>[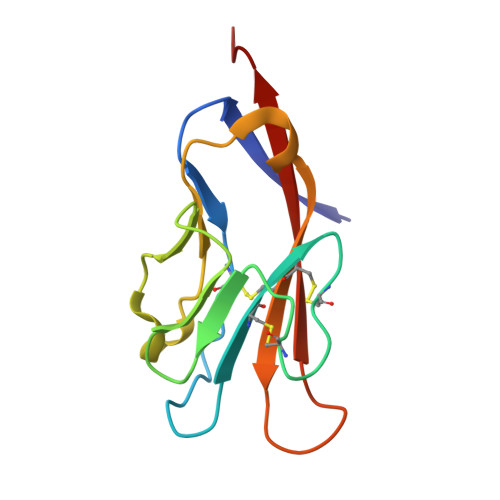2x]SETVVTEVLGHRVTLPCLYSSWSHNSNSMCWGKDQCPYSGCKEALIRTDGMRVTSRKSAKYRLQGTIPRGDVSLTILNPSESDSGVYCCRIEVPGWFNDVKINVRLNLQRALV>PPPLSHCGRAAPCEPLRYNVCLGSVLPYGATSTLLAGDSDSQEEAHGKLVLWSGLRNAPRCWAVIQPLLCAVYMPKCENDRVELPSRTLCQATRGPCAIVERERGWPDFLRCTPDRFPEGCTNEVQNIKFNSSGQCEVPLVRTDNPKSWYEDVEGCGIQCQNPLFTEAEHQDMHSYIAAFGAVTGLCTLFTLATFVADWRNSNRYPAVILFYVNACFFVGSIGWLAQFMDGARREIVCRADGTMRLGEPTSNETLSCVIIFVIVYYALMAGVVWFVVLTYAWHTSFKALGTTYQPLSGKTSYFHLLTWSLPFVLTVAILAVAQVDGDSVSGICFVGYKNYRYRAGFVLAPIGLVLIVGGYFLIRGVMTLFSIKSNHAKALIVYGSTTGNTEYTAETIARELADAGYEVDSRDAASVEAGGLFEGFDLVLLGCSTWGDDSIELQDDFIPLFDSLEETGAQGRKVACFGCGDSSWEYFCGAVDAIEEKLKNLGAEIVQDGLRIDGDPRAARDDIVGWAHDVRGAIKINETMLRLGIFGFLAFGFVLITFSCHFYDFFNQAEWERSFRDYVLCQANVTIGLPTKQP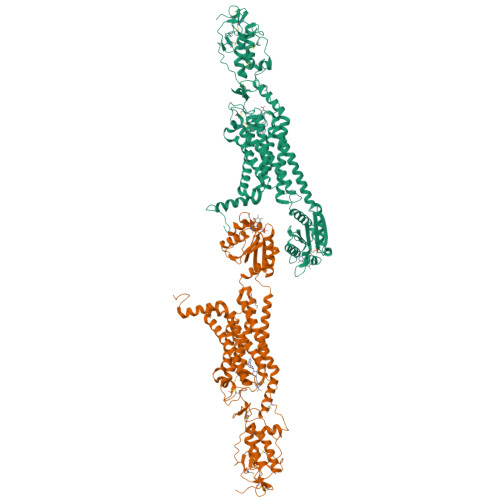IPDCEIKNRPSLLVEKINLFAMFGTGIAMSTWVWTKATLLIWRRTWCRLTGQSDDHHHHHHHHHH[2x]> GSPLPWCPHLVAVCPIPAAGLDVTQPCGDCGTIQENWVCLSCYQVYCG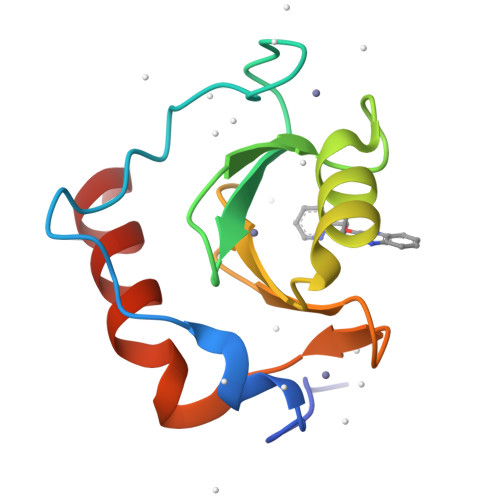RYINGHMLQHHGNSGHPLVLSYIDLSAWCYYCQAYVHHQALLDVKNIAHQNKFG> GSKKHSVLHLVPVNITSKADSDVTEVMWQPVLRRGRGLEAQGDIVRVWDTGIYLLYSQVLFHDVTFTMGQVVSREGQGRRETLFRCIRSMPSDPDRAYNSCYSAGVFHLHQGDIITVKIPRANAKLSLSP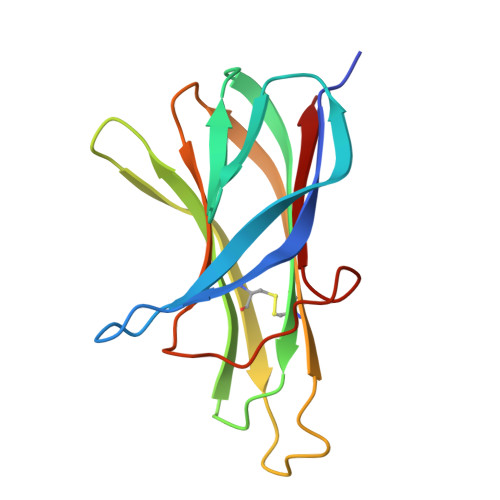HGTFLGFVKL>[2x]ETLVRPKPLLLKLLKSVGAQKDTYTMKEVLFYLG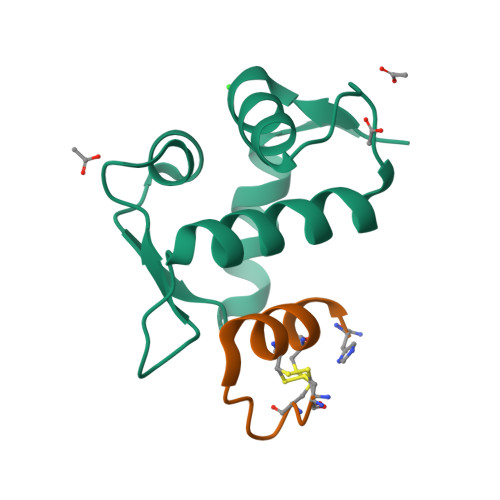QYIMTKRLYDEKQQHIVYCSNDLLGDLFGVPSFSVKEHRKIYTMIYRNLVV;>CNCKAPETFLCYWRCLQH[2x]>AEGDDPAKAAFDSLQASATEMIGYAWAMVVVIVGATIGIKLFKKFTSKAS[75x]

Most extensively studied in this group are the F-specific filamentous phages (Ffs) that include viruses f1, fd and M13. Ffs are also strikingly simple—their single-stranded DNA genome encodes just 11 proteins, of which 5 form the phage capsid. pVIII is the major capsid protein that forms the filamentous body of the phage. The tips of the filament are formed of the minor capsid proteins which occur in pairs. pIII and pVI form the leading end of the infecting phage, which interacts with the host receptors to initiate entry, whereas pVII and pIX form the trailing end11,12.

pVIII forms the main body of the filamentous phage. It is produced initially with a signal sequence that is cleaved to leave a single α-helix of 50 residues in length, with thousands of these helices packing together in a helical array to coat the length of the phage DNA genome. The α-helices are slightly curved; with their C-termini projecting into the phage lumen, resulting in an overall highly positive charge. The N-terminus of pVIII is splayed outwards towards the exterior of the capsid. In our map, density is smeared for the four N-terminal residues, indicating that these are flexible. The helical parameters were determined using cryoSPARC and were refined to a helical twist of 37.44° and a helical rise of 16.6 Å. In the filamentous section, pVIII interacts with its neighbours by mainly hydrophobic interactions, with hydrogen bonds observed at the C-termini and mostly involving lysine residues. The positively charged lumen of the virion is comprised mainly of lysine residues from the C-terminal ends of pVIII molecules, hence allowing them to interact with the negatively charged DNA molecule. Four lysine residues from each pVIII monomer (Lys 40, 43, 44 and 48) line the DNA cavity. Overlaying a protomer of our f1-derived nanorod pVIII with a previously determined fd phage pVIII structure (2C0W; determined by X-ray fibre diffraction) shows that the two are broadly similar (RMSD of 1.0 Å across 39 pruned pairs; RMSD of 1.5 Å across all 46 pairs).OCTANE-1,8-DIOL | C8 H18 O2 | 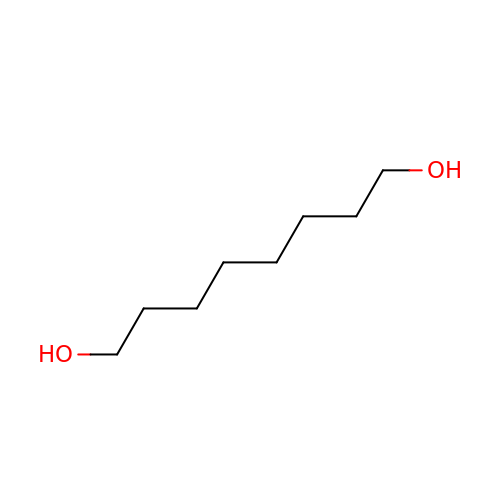OEIJHBUUFURJLI-UHFFFAOYSA-N>MMKRNILAVIVPALLVAGTANAAEIYNKDGNKVDLYGKAVGLHYFSKGNGENSYGGNGDMTYARLGFKGETQINSDLTGYGQWEYNFQGNNSEGADAQTGNKTRLAFAGLKYADVGSFDYGRNYGVVYDALGYTDMLPEFGGDTAYSDDFFVGRVGGVATYRNSNFFGLVDGLNFAVQYLGKNERDTARRSNGDGVGGSISYEYEGFGIVGAYGAADRTNLQEAQPLGNGKKAEQWATGLKYDANNIYLAANYGETRNATPITNKFTNTSGFANKTQDVLLVAQYQFDFGL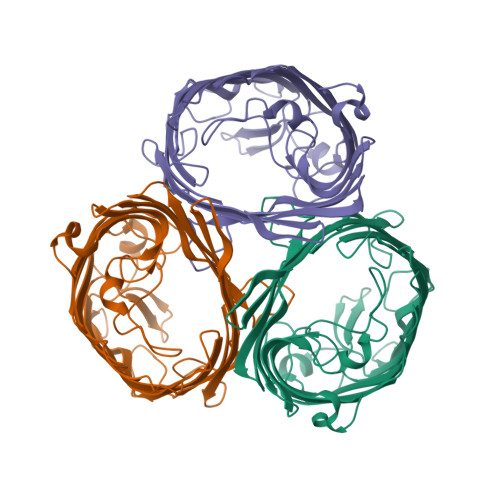RPSIAYTKSKAKDVEGIGDVDLVNYFEVGATYYFNKNMSTYVDYIINQIDSDNKLGVGSDDTVAVGIVYQF[6x]[(6E,11E)-2,6,12,16-tetramethylheptadeca-2,6,11,15-tetraene-9,9-diyl]bis(phosphonic 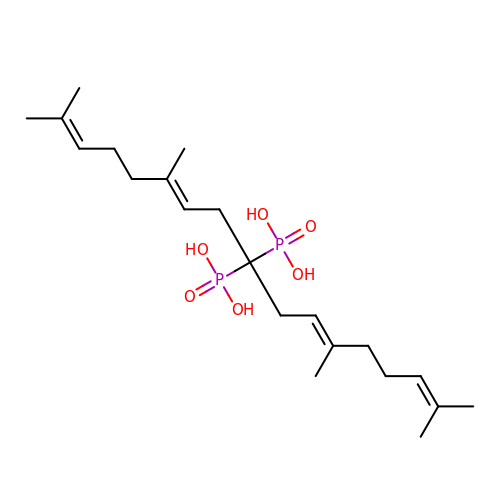acid) | C21 H38 O6 P2 | SQERRIVHBWCION-IWGRKNQJSA-N>[5x]MGGELEKVKAEALAVLAAIGSPAAKFA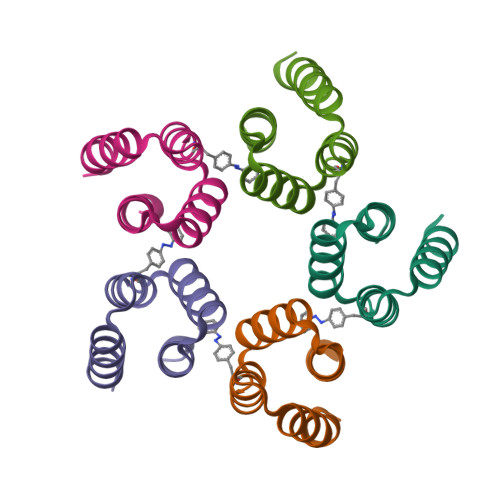VEAVERDHFSAIEIAARFLLEIGDEEGSRVLLEYSDVLRKHHHHHH> MGDVRLSALSTLNYRNLAPGTLNFPEGVTGIYGENGAGKTNLLEAAYLALTGQTDAP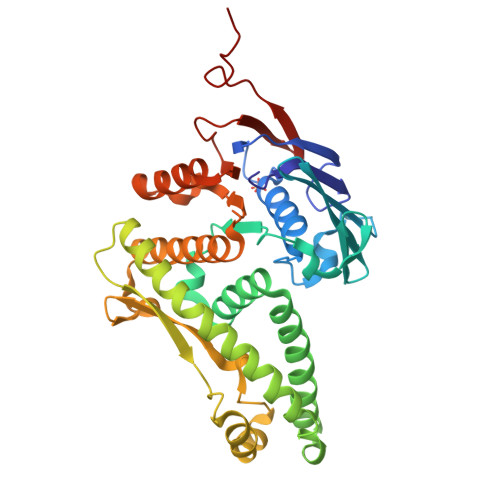RIEQLIQAGETEAYVRADLQQGGSLSIQEVGLGRGRRQLKVDGVRARTGDLPRGGAVWIRPEDSELVFGPPSGRRAYLDSLLSRLSARYGEQLSRYERTVSQRNAALRGGEEWAMHVWDDVLLKLGTEIMLFRRRALTRLDELAREANAQLGSRKTLALTLTESTSPETYAADLRGRRAEELARGSTVTGPHRDDLLLTLGDFPASDYASRGEGRTVALALRRAELELLREKFGEDPVLLLDDFTAELDPHRRQYLLDLAASVPQAIVTGTELAPGAALTLRAQAGRFTPVADEEMQAEGTA> GSPGISGGGGGSHIEGYECQPIFLNVLEAIEPGVVCAGHDNNQPDSFAALLSSLNELGERQLVHVVKWAKALPGFRNLHVDDQMAVIQYSWMGLMVFAMGWRSFTNVNSRMLYFAPDLVFNEYRMHKSRMYSQCVRMRHLSQEFGWLQITPQEFLCMKALLLFSIIPVDGLKNQKFFDELRMNYIKELDRIIACKRKNPTSCSRRFYQLTKLLDSVQPIARELHQFTFDLLIKSHMVSVDFPEMMAEIISVQVPKILSGKVKPIYFHTQ;> SRFADFFRNEGLGSRSGSGK

The androgen receptor (AR) is the cellular mediator of the actions of the hormone 5-α dihydrotestosterone (DHT). Androgen binding to AR leads to activation of genes involved in the development and maintenance of the male reproductive system and other tissues such as bone and muscle. AR is distinguished from other nuclear receptors in that after hormone binding, it preferentially responds to a specialized set of coactivators bearing aromatic-rich motifs, while responding poorly to coactivators bearing the leucine-rich “NR box” motifs favored by other nuclear receptors. Structures of AR in complex with FxxLF, LxxLL, FxxLW, WxxLF, WxxVW, FxxFF, and FxxYF motifs reveal a changing surface of the AR coactivator binding interface that permits accommodation of both AR-specific aromatic-rich motifs and canonical leucine-rich motifs.

Finally, effects of substitutions at the +4 position were assessed in structures of AR in complex with peptides containing FxxFF and FxxYF motifs. Surprisingly, the binding mode of FxxFF to AR resembled that of the tryptophan peptides more closely than the binding mode of FxxLF. Like the tryptophan peptides, interactions with Glu897 are mediated by Ser−2 instead of the peptide backbone. Deviations from ideal helical geometry allow Phe+4 to bind facedown in the +4 pocket with the benzyl ring stacked against Val713. With the exception of FxxFF, motifs containing phenylalanines at the +1 and +5 positions present canonical main chain interactions with both charge clamp residues, Lys720 and Glu897.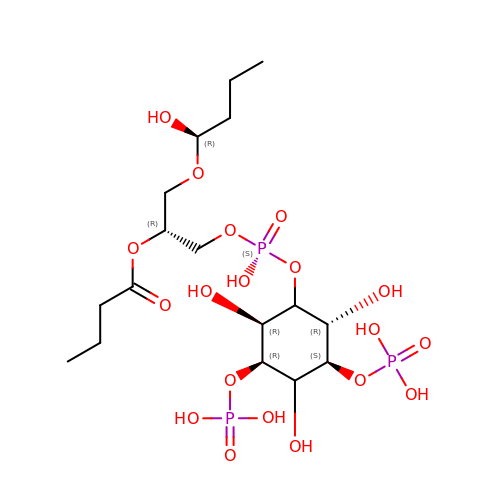(1S)-2-(1-HYDROXYBUTOXY)-1-{[(HYDROXY{[(2R,3S,5R,6S)-2,4,6-TRIHYDROXY-3,5-BIS(PHOSPHONOOXY)CYCLOHEXYL]OXY}PHOSPHORYL)OXY]METHYL}ETHYL BUTYRATE | C17 H35 O19 P3 | SEWBGVDZVBOXHU-DSHZNZJQSA-N>MRGSHHHHHHGSMAEGEEYDKILVLNFGSQYFHLIVKRLNNIKIFSETKDYGVELKDIKDMNIKGVILSGGPYSVTEAGSPHLKKEVFEYFLEKKIPIFGICYGMQEIAVQMNGEVKKSKTSE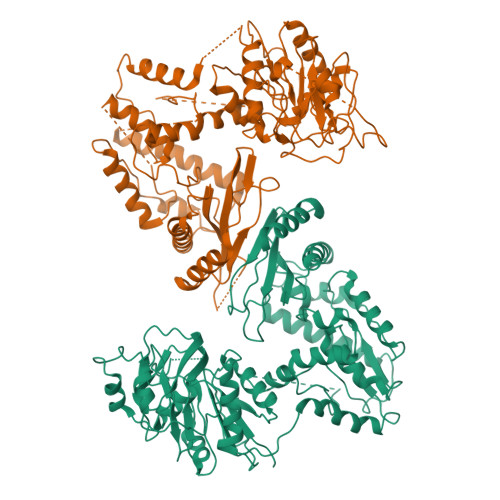YGCTDVNILRNDNINNITYCRNFGDSSSAMDLYSNYKLMNETCCLFENIKSDITTVWMNHNDEVTKIPENFYLVSSSENCLICSIYNKEYNIYGVQYHPEVYESLDGELMFYNFAYNICKCKKQFDPIRYHELELKNIEKYKHDHYVIAAMSGGIDSTVAAAYTHKIFKERFFGIFIDNGLLRKNEAENVYTFLKSTFPDMNITKIDASENFLSNLQGVTDPEQKRKIIGKLFIEEFEKAVNNIDIDINKTFLLQGTLYPDIIESKCSKNLSDTIKTHHNVGGLPKNLKFKLFEPFKYLFKDDVKTLSRELNLPEEITNRHPFPGPGLAIRVIGEINKHKLNILREVDDIFINDLKQYGLYNQISQAFAVLLSSKSVGVRGDARSYDYVCVLRAVKTSSFMTANWYQIPYDILDKITTRILSEVKGVNRILYDVSSKPPATIEFE[2x]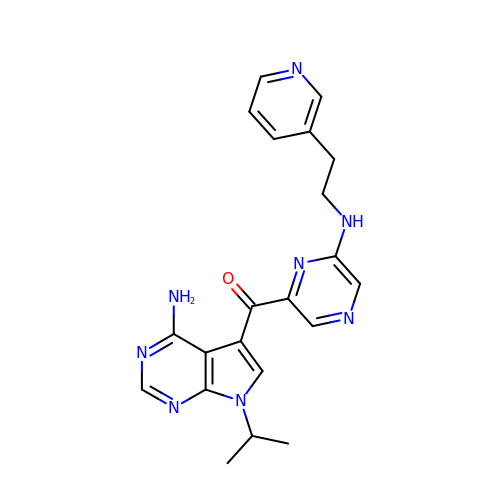[4-amino-7-(propan-2-yl)-7H-pyrrolo[2,3-d]pyrimidin-5-yl](6-{[2-(pyridin-3-yl)ethyl]amino}pyrazin-2-yl)methanone | C21 H22 N8 O | WMUOCKJUZCEMCY-UHFFFAOYSA-N>[2x]VEDEFSYIDGNPNGPENWGNLK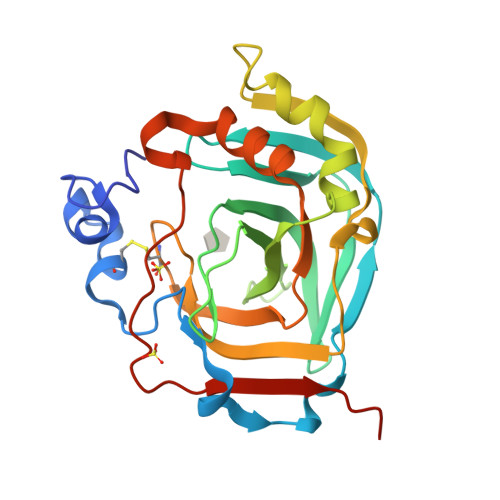PEWETCGKGMEQSPIQLRDNRVIFDQTLGKLRRNYRAVDARLRNSGHDVLVDFKGNAGSLSINRVEYQLKRIHFHSPSEHEMNGERFDLEAQLVHESQDQKRAVVSILFRFGRADPFLSDLEDFIKQFSNSQKNEINAGVVDPNQLQIDDSAYYRYMGSFTAPPCTEGISWTVMRKVATVSPRQVLLLKQAVNENAINNARPLQPTNFRSVFYFEQLKSKLGVI>[2x]GAMPHDPSFTPTQLAARAAYLLRGN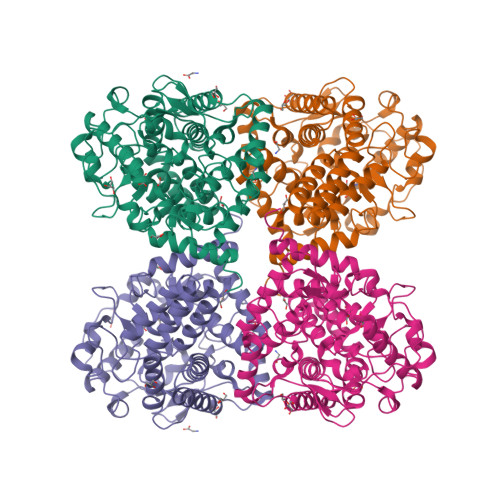DLGTMTTAAPLLYPHMWSWAAAFVAIGLAPLSVERAVVELDTLLSAQWRNGMIPHIVFANGVDGYFPGPARWATATLADNAPRNRLTSGITQPPVHAIAVQRILEHARTRGRSTRAVAEAFLDRRWGDLMRWHRWLAECRDRNERGRITLYHGWESGMDNSPRWDSAYANVVPGKLPEYQRADNVIITDPSQRPSDGEYDRYLWLLEEMKAVRYDDERLPSVMSFQVEDVFFSAIFSVACQVLAEIGEDYKRPHADVKDLYLWAERFRAGVVETTDQRTGAARDFDVLAEKWLVTETAAQFAPLLCGGLPHDRERALLKLLEGPRFCGHPDLKYGLIPSTSPVSRDFRPREYWRGPVWPVLTWLFSWCFARRGWAERARLLRQEGLRQASDGSFAEYYEPFTGEPLGSMQQSWTAAAVLDWLG>HMGSMALDGIRMPDGCYADGTWELSVHVTDLNRDVTLRVTGEVHIGGVMLKLVEKLDVKKDWSDHALWWEKKRTWLLKTHWTLDKCGIQADAKLQFTPQHKLLRLQLPNMKYVKVKVNFSDRVFKAVSDICKTFNIRHPEELSLLKKPRDPTKKKKKKLDDQSEDEALELEPGILAVSQPVTSPEILAKMFKPQALLDKAKTNQGWLDSSRSLMEQDVKENEALLLRFKYYSFFDLNPKYDAIRINQLYE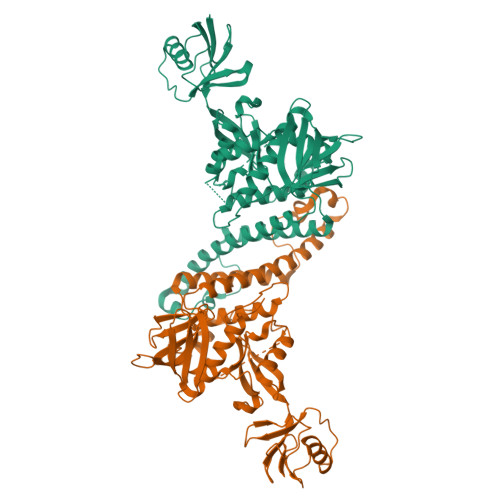QAKWALLLEEIECTEEEMMMFAALQYHINKLSIMTSENHLTTDVNPECLVSPRYLKKYKSKQITARILEAHQNVAQMSLIEAKMRFIQAWQSLPEFGITHFIARFQGGKREELIGIAYNRLIRMDASTGDAIKTWRFSNMKQWNVNWEIKMVTVEFADEVRLSFICTEVDCKVVHEFIGGYIFLSTRAKDQNESLDEEMFYKLTSGWV[2x]> GAMAFDWDAYLEETGSEAAPAKCFKQAQNPPNNDFKIGMKLEALDPRNVTSTCIATVVGVLGSRLRLRLDGSDSQNDFWRLVDSTEIHAIGHCEKNGGMLQPPLGFCMNASSW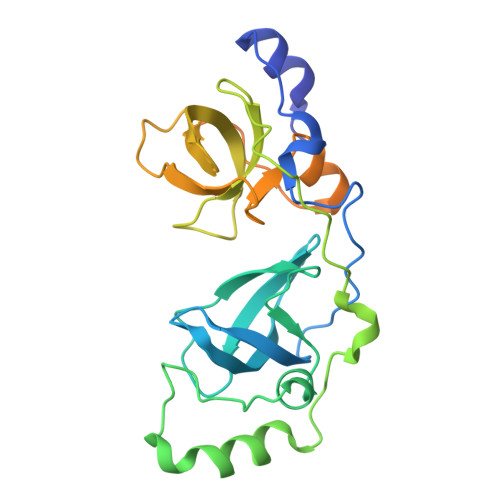PGYLCKILNNAMVAPEEIFQPEPPEPEENLFKVGQKLEAVDKKNPQLICCATVDAIKDDQIHVTFDGWRGAFDYWCNYRSRDIFPAGWCARSCHPMQPPGHKSRMDSSSSKQRCPRPRYTVVAESEAMVPASPATAHFHPNCKGGPFINNSK>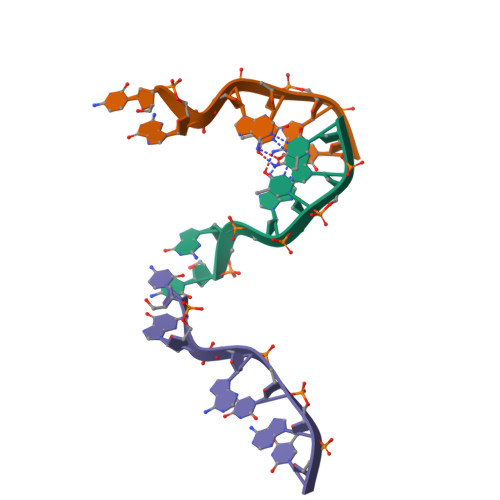 CGATAT>[2x]MKKRVVKLRELVPAVAALAVAVLIQSATGSSGGSGHTPTTQATHADDHDLTTHNGTEEHDDGHDDGHDDLHAHAPKVIVFISGSCLFGAISRSLFKKLPIPYTVVLLILGAILGVVASNVPLVEEHTRDVAHMDPHVLLQIFLPVLIFESAFAMDVHTFMRSFSQVCILALFGLVVASVLTAVLAMNLFNYNWNFSEAMMFGAIMSATDPVAVVALLKDLGASKQLGTIIEGESLLNDGCAIVIFNVFMKMVFFPQLTSTVGQNVLYFLQVAVAGPLWGYAVAKVTVFFLSHIFNDALVEITITLAATYLTYYIGDIWLEVSGVLAVVVLGLIVNAEKTSISPEVEVFLHRFWEMLAYLANTLIFMMVGVVVTQKALVAVDKMDWFYLIILYLAITIIRGMVISLFSPILSRIGYGLTWRNAVIMTWGGLRGAVGLALALVVENLAGNDVIGSKFLFHTAGIVVLTLVINATTIQTLLRILGMSDISIPKRLAMAGAVRRIHEGQNRTLNMLKSDRFLADADWDIATAACEISDPYSALSDDENAPADELTLGERKSVCPGCKAMVPNEPSPREFADMMEEARLRMLKAEKISYWKQFEHGMLAREALRLLVQHAEVAADEKDQFILVDDLKKSWQIKGIYPWLKRKLEDLISEKKIAAIPMPKYKLGKLMYKICHHMAFEVTINIAIVLNIVPIIMEFVV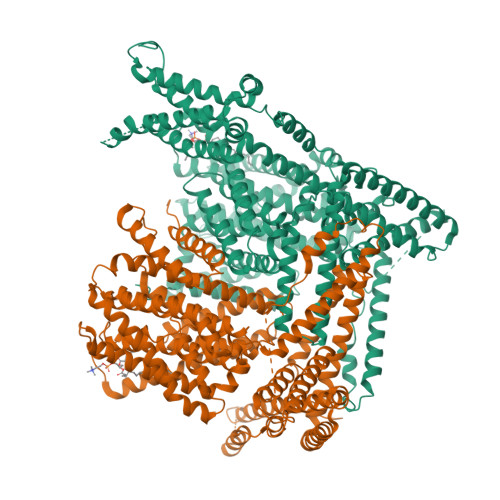QDKMASVSTMAAPGSTVSSEPSSLQKIEDALRISNYVFFVIYAIEAIVKILGLGRHYIVSHWNKFDAFILVVALVDIIIAETLLKGSITINLSSIKVVKLFRLLRGLRMLRLTKALIPKLILVVNGKINNQLSLGYDVGKGYIIGEEEVGKIIDRMVDNKKILRELKHISETGRLQVVKELGLLQREHPGIAVSVKTRQAIRTILNHSRETIHELQGAGLLDEMEAHKLELTVEIKMKRLMNAPSSIPPPPPENLLKNVSWLAGDMKLIDFIKARASLLHFDYGEVIVREGDESDGLFLIVSGLVKLYGKSAFLDHDNPPVTAGSEENEVFEDYLTVGNVIGEMGVLTKKPRNATVTCETTVQVYFITAEDMNIAIDTFTLYPSLEYRLWRVVAIRIATPLIMEQMAFQGWTQEKVKLHLERGYLVDLAESHFQFNIDATLEDVILINGTAYNAHTREEIRSPCLISRTVHKLTFQYTATEEPRLFVVRNAEYNGPILDGRLDVDSKRSLISITEISSNMCLKHAAELRQKNSKVMLSRKSSGAAAKEEEDCIPNTSDVEQAAGVSPSVPTKTTPKPKSFLPSLGLSMSKERVNGEAVEESPVKTKQGEETPETEEGAAPRVNVENLYFQ> DRHHHHHHKLDRKPRHYEINLDEPPSQRWNQVIKDHLEYLPGVVE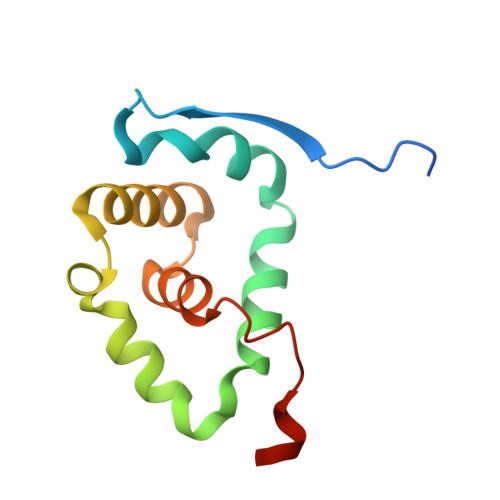ETKKYIPKPLQPFVWWAASKIDRYFTTEIQEELKGIASESGLPIGEIVGMNILYDVAAFDRRHIFGLG> MLEQPYLDLAKKVLDEGHFKPDRTHTGTYSIFGHQMRFDLSKGFPLLTTKKVPFGLIKSELLWFLHGDTNIRFLLQHRNHIWDEWAFEKWVKSDEYHGPDMTDFGHRSQKDPEFAAVYHEEMAKFDDRVLHDDAFAAKYGDLGLVYGSQWRAWHTSKGDTIDQLGDVIEQI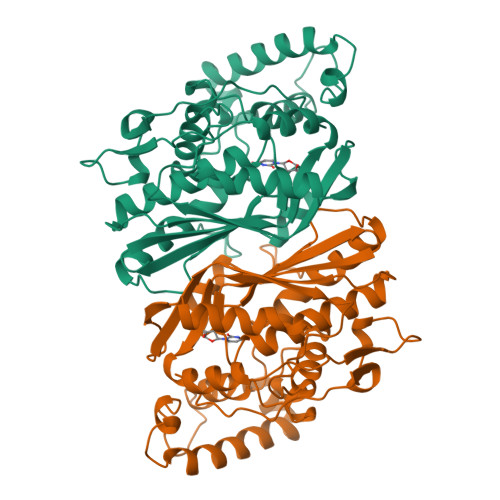KTHPYSRRLIVSAWNPEDVPTMALPPCHTLYQFYVNDGKLSLQLYQRSADIFLGVPFSIASYALLTHLVAHECGLEVGEFIHTFGDAHLYVNHLDQIKEQLSRTPRPAPTLQLNPDKHDIFDFDMKDIKLLNYDPYPAIKAPVAV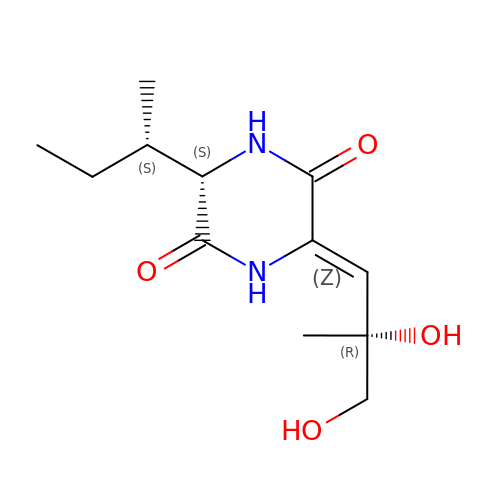(3S,6Z)-3-[(2S)-butan-2-yl]-6-[(2R)-2-methyl-2,3-bis(oxidanyl)propylidene]piperazine-2,5-dione | C12 H20 N2 O4 | KGPSCQPJVWXIGR-PMSMWWAASA-N>SNAMRHDEYQYLDLIRQIMRTGNRKGDRTGTGTISMFGAQMRYSLRDGI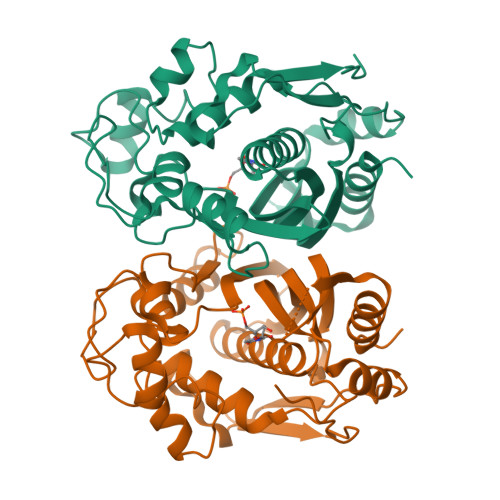FPLLTTKRVFWRGVAEELLWFVRGSTNAKELQEKDIHIWDGNSSKEFLNKMGFHDREEGDLGPVYGFQWRHFGAPYADMHTDYTGQGVDQLQQVIDTIKNNPDDRRIIMCAWNPVDVPKMALPPCHCLCQFYVANGELSCQLYQRSADMGLGVPFNIASYALLTYMIAHVTDLKPGDFVHTLGDAHVYSNHCEALEEQLKREPRPFPSLKIKRKVENISDFKFEDFELDGYKPHPKIKMEMAV[2x]> KEVCYERLGCFSDDSPWSGITERPLHILPWSPKDVNTRFLLYTNENPNNFQEVAADSSSISGSNFKTNRKTRFIIHGFIDKGEENWLANVCKNLFKVESVNCICVDWKGGSRTGYTQASQNIRIVGAEVAYFVEFLQSAFGYSPSNVHVIGHSLGAHAAGEAGRRTNGTIGRITGLDPAEPCFQGTPELVRLDPSDAKFVDVIH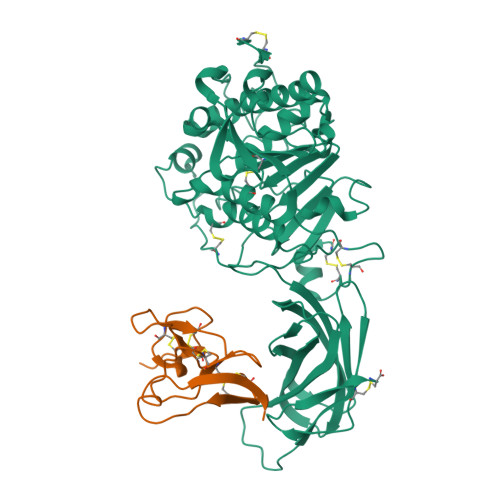TDGAPIVPNLGFGMSQVVGHLDFFPNGGVEMPGCKKNILSQIVDIDGIWEGTRDFAACNHLRSYKYYTDSIVNPDGFAGFPCASYNVFTANKCFPCPSGGCPQMGHYADRYPGKTNDVGQKFYLDTGDASNFARWRYKVSVTLSGKKVTGHILVSLFGNKGNSKQYEIFKGTLKPDSTHSNEFDSDVDVGDLQMVKFIWYNNVINPTLPRVGASKIIVETNVGKQFNFCSPETVREEVLLTLTPC;> VPDPRGIIINLDEGELCLNSAQCKSNCCQHDTILSLLRCALKARENSECSAFTLYGVYYKCPCERGLTCEGDKSLVGSITNTNFGICHNVGRSDS>PSSETFVFTKDNLVGNTQGSFTFGPSLSDCPAFKDGILKAYHEYKIT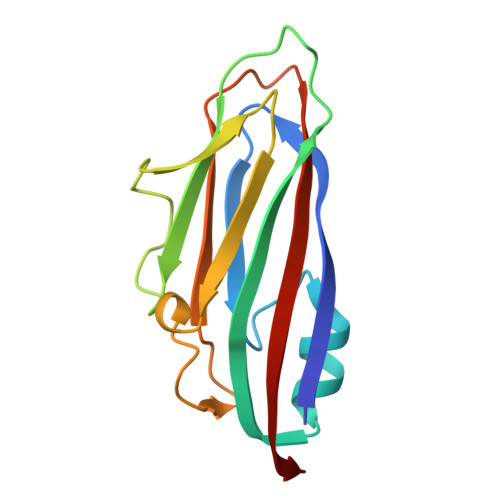SILLQFVSEASSTSSGSIAYELDPHCKVSSLQSYVNKFQITKGGAKTYQARMINGVEWHDSSEDQCRILWKGNGKSSDPAGSFRVTIKVALQNPK[6x]>[4x]DSIIHIGAIFEENAAKDDRVFQLAVSDLSLNDDILQSEKITYSIKVIEANNPFQAVQEACDLMTQGILALVTSTGCASANALQSLTDAMHIPHLFVQRNPGGSPRTACHLNPSPDGEAYTLASRPPVRLNDVMLRLVTELRWQKFVMFYDSEYDIRGLQSFLDQASRLGLDVSLQKVDKNISHVFTSLFTTMKTEELNRYRDTLRRAILLLSPQGAHSFINEAVETNLASKDSHWVFVNEEISDPEILDLVHSALGRMTVVRQIFPSAKDNQKCMRNNHRISSLLCDPQEGYLQMLQISNLYLYDSVLMLANAF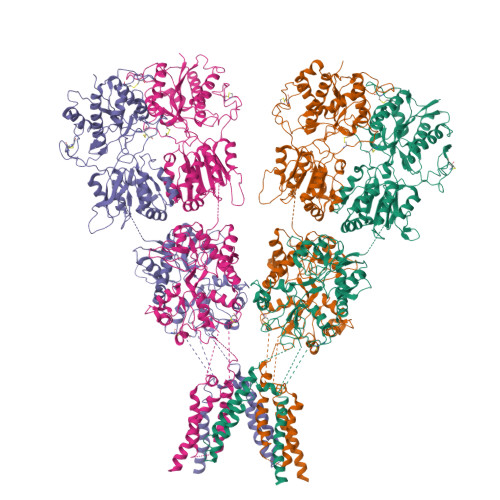HRKLEDRKWHSMASLNCIRKSTKPWNGGRSMLDTIKKGHITGLTGVMEFREDSSNPYVQFEILGTTYSETFGKDMRKLATWDSEKGLNGSLQERPMGSRLQGLTLKVVTVLEEPFVMVAENILGQPKRYKGFSIDVLDALAKALGFKYEIYQAPDGRYGHQLHNTSWNGMIGELISKRADLAISAITITPERESVVDFSKRYMDYSVGILIKKPEEKISIFSLFAPFDFAVWACIAAAIPVVGVLIFVLNRIQAVRSQSATQPRPSASATLHSAIWIVYGAFVQQGGESSVNSVAMRIVMGSWWLFTLIVCSSYTANLAAFLTVSRMDSPVRTFQDLSKQLEMSYGTVRDSAVYEYFRAKGTNPLEQDSTFAELWRTISKNGGADNCVSNPSEGIRKAKKGNYAFLWDVAVVEYAALTDDDCSVTVIGNSISSKGYGIALQHGSPYRDLFSQRILELQDTGDLDVLKQKWWPHTGRCDLTSHSSAQTDGKSLKLHSFAGVFCILAIGLLLACLVAALELWWNSNRCHQETPKEDKEVGLVPR phenacyl coenzyme A | C29 H42 N7 O17 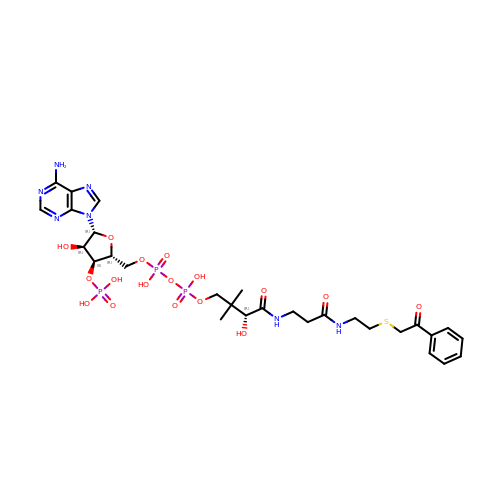P3 S | WOEFYXMDPBOUAP-VXAHOBLNSA-N> MKKNFFHLLIMLICSYISFAYANISDYRVMTWNLQGSSASTESKWNINVRQLLSGTAGVDILMVQEAGAIPTSAVRTGRHIQPF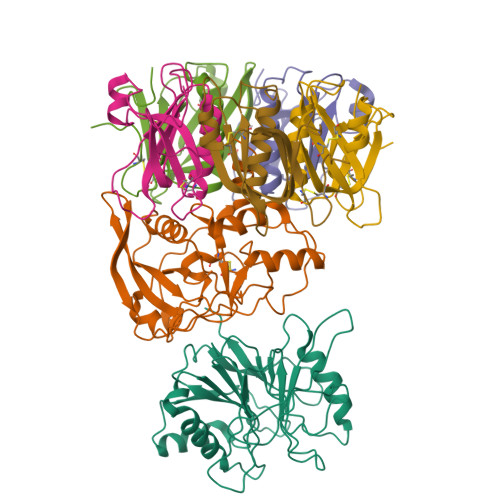GVGIPIDEYTWNLGTTRRQDIRYIYYSPIDVGARRVNLAIVTRRRADNVYVLRPTTVASRPIIGIGLGNDVFLTTHALASGGPDAAAIVRVTYNFFRTPQMRHLSWLLGGDFNRAPDRLESDLMTEHLERLVTIIAPTEPTQIGGNILDYGVIVDRAPYSQRVEALRNPQLASDHYPVAFEAQHCG;> MKKLILLTLIIASFDIYAIDFVYRVDPNPPDVIFRDGFSLLGYNRDLQQLISGRSCAGGSSDSRYIVTTSDINKTYAIARAYYSHSKFKGNLYRYKIRADNNFYSLTPSVNYLESQGGHFNAYEKSMIRLQSEYVSTLSILPENIQKAVALVYDSSTGQIKDGTSTINTDYVSISSVSNPGVIPFLPEPQANTQQRIDAFGSLISSCFSIYSVCQTHRGQKTEVYKMPFYDARPVIQFIISGN;>[3x]MKKITSVCALLSLICSFNASAEWTGDYENIGYFSHEVISEFHVGQIDGGAYFCIKAVKADGSRSTPLIACSVSNESVWAPSFKVLLEQARYFYVTEQSVRIYYDHNVWTNQPFVNTFSTNALVGLSSCSAATDCFGPGKPKSKSKRDVEQ;>[2x]EWTGDSSINYYSDEVISDFHVGQFNRSAYFCIKTVKKSGEGTPIIACALSHDSKWIPSFNIMLEQARNFYITGHSIRVYVQPNVWSNKSFIEALSSNALVGLSSCSTSECFGPVKP> GSDPTQFEERHLKFLQQLGKGNFGSVEMCRYDPLQDNTGEVVAVKKLQHSTEEHLRDFEREIEILKSLQHDNIVKYKGVCYSAGR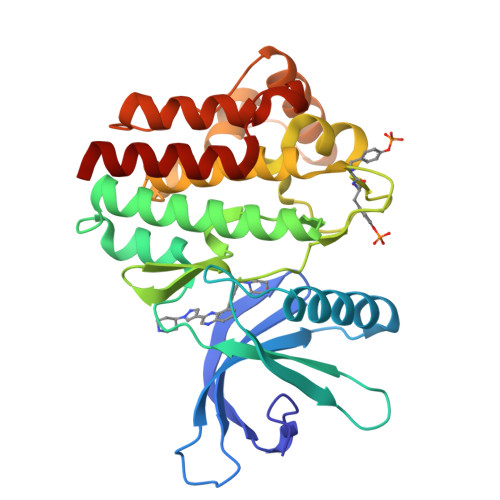RNLKLIMEYLPYGSLRDYLQKHKERIDHIKLLQYTSQICKGMEYLGTKRYIHRDLATRNILVENENRVKIGDFGLTKVLPQDKEYYKVKEPGESPIFWYAPESLTESKFSVASDVWSFGVVLYELFTYIEKSKSPPAEFMRMIGNDKQGQMIVFHLIELLKNNGRLPRPDGCPDEIYMIMTECWNNNVNQRPSFRDLALRVDQIRDNMAG> MLQKKPY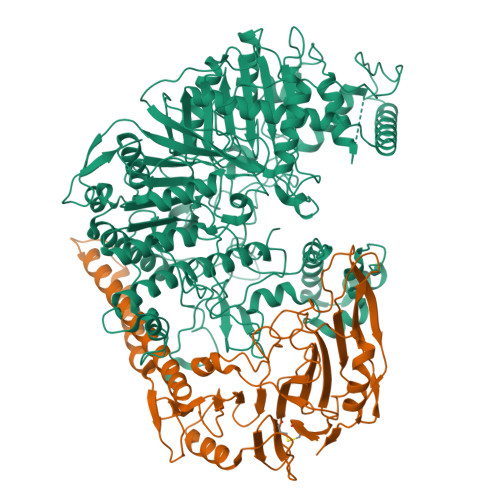NGLHEKELNQINQQDGSPCVAISAPGCFIKGSNLFSEKRAGNRVRFFTTGRDYFSDLASALDSASSSIFITGWQVNYDVLLDGRRSLWQCLRQALERSPALKVYVMPWLSPSGSLGTYDFETMLAVFQLNAGLEGGARAFCTPAIQQSDMQGLGVAFSHHQKSVVIDNRIGYVGGIDLAYGRRDDNDFSLDASGRRGNDAYNPGLPHLGWMAEDEHVSSMGLMMATLFDLSRPLASLTLHAPTLRLSPFPHIAASDEPLLSIPLAPSRARALNGAAYLSDLFRSPMLPSLQWLGRAYNSSKEGLDEGFERLDALRRQMVASSIRAIANLIADNLDALPIEPELERRLRAWLEELRTAALNLPEALRIKSLLLINQWMSETELGQVLTLISGKGFEDIPQNLSGKAGELAGSLFWTLHRLMQARAGGHQQPYRYLDEAPQPLASPDNARLAADQPRMPWQDVHCRIEGPSVYDLARNFIDRWNGQQAYLAKTPALQDTALVRSALEAVMKWLNSLAAAAGLENYLDEKRNLRLELDPPTPCWINAPEQLPQEPEVRRGGMTVQVLRSAAARMLEQEQAGRLGAGVNLPLQVGVSTEGVQSNCKDAMLLAISGAQQFIYIENQFFQSEFGKEGEVFKDLPLSGPMASLRDVGSLRRDFVVRIRLEEALEQRDLWLLDWAEVEKIAQEPGTEARQFLKSMLAMWGVNAQGWLTHKLGEAQHGLLNEIGEALARRIERAIQREHPFHVYLVLPVHPEGALNVPNIMHQVHLTQQSLVFGEQSLVKRIQRQMALKALEGKSDPAQAREIIERKDARGRPVYEQQDWSRYLTLLNLRTWAVLGGRVVTEQIYVHSKLLIADDRVAILGSANINDRSLQGERDSELAVMVRDSEPLTVRLDGKNDAIVGKAIHQLRVNLWKKHFGLSQGPGGFVKPASELSAYLSIPAAQEAWEAIQTLAKENTRAYERTFNFIPQNISQTQLQLTPEPPKGFEDGFPASIWPTWAYRKPGELRAGGQLMEPMPYQEIFWRSSNLTSVKTFPPPNGVSGFITALPTSWTRGERNDSGLNLSILAHQDSRSLPTQVAMNGDSSAQGKHRT;> MKRVLMGLILLSSSNITWAEAPSSKYQECLGRMTFEIPEEMEWATYDASRVWQISKGGGHNFTAEVTAVGDNGSYDYDSMIFYVSEKVDKNEFHNASNYIKGTAEIYQDHLRENIKLDKKAISTLQKNKSEEKSIERIKKGIAEMEAKIPLAKIYEHDLGIPDSHILGSKNIPFHVLLWRNQRVYYFTFSKPTENSAQRIKDLIARFRTRELYEVPNEPGICFPYGFIADDGKTAYELKNSLRFTRTPNVIFSLLTASANDPWQTRPTSGLYDSDFRPGYDRQKWKKSALLDSLHIGKRLAAFEGWRLDPRPDSGERERAWFGLAHTGGTLDPLVAIQVQTFQKGTDDLTDYTPPPEEVLPRLKALSQSIEQRLAR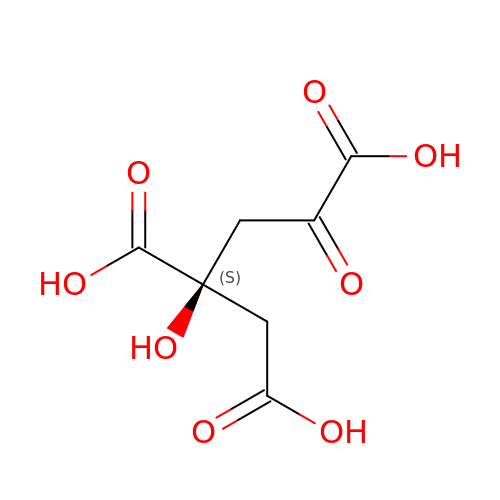(2S)-2-hydroxy-4-oxobutane-1,2,4-tricarboxylic acid | C7 H8 O8 | RQMCNDRMPZBEOD-ZETCQYMHSA-N>[2x]GSKKIFKPEELRQALMPTLEAL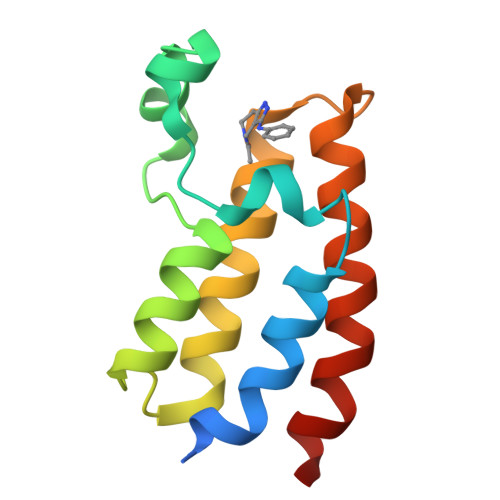YRQDPESLPFRQPVDPQLLGIPDYFDIVKNPMDLSTIKRKLDTGQYQEPWQYVDDVWLMFNNAWLYNRKTSRVYKFCSKLAEVFEQEIDPVMQSLG> GGGSGGGSKFADHLHKFHENDNGA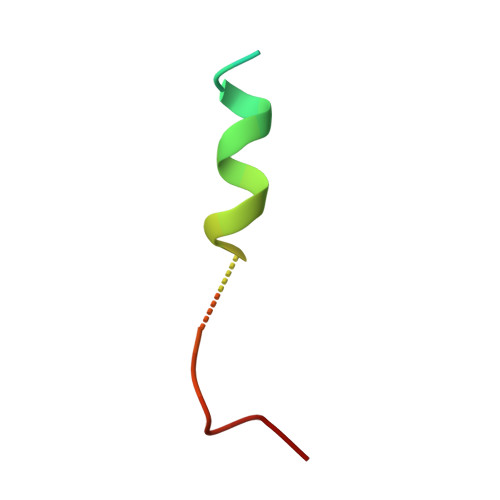AAGDLWQ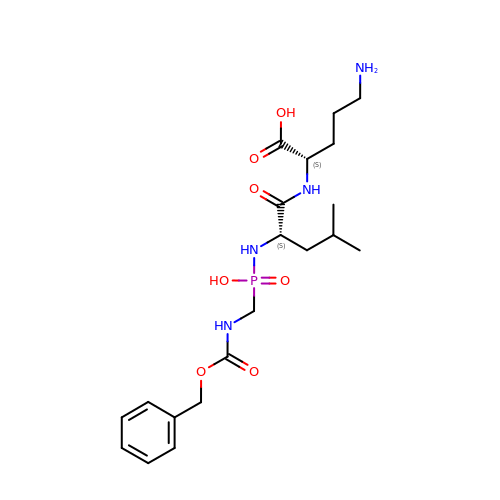(2~{S})-5-azanyl-2-[[(2~{S})-4-methyl-2-[[oxidanyl(phenylmethoxycarbonylaminomethyl)phosphoryl]amino]pentanoyl]amino]pentanoic acid | C20 H33 N4 O7 P | WVIBWHYQVPNZPE-IRXDYDNUSA-N>[3x]MESDDLMNDPRASNTNLIVNYLPQDMTDRELYALFRAIGPINTCRIMRDYKTGYSFGYAFVDF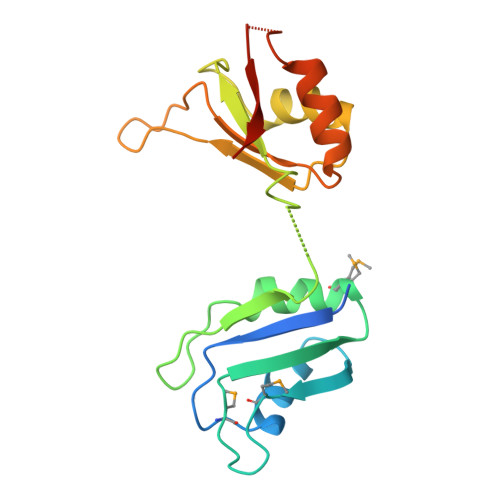TSEMDSQRAIKVLNGITVRNKRLKVSYARPGGESIKDTNLYVTNLPRTITDDQLDTIFGKYGSIVQKNILRDKLTGRPRGVAFVRYNKREEAQEAISALNNVIPEGGSQPLSVRLAEEHGK> GAMAVKVARPCRKIEKWTYLELKGSKANEGVPQAMTAFAEFLNRTGIPINPRFSPGMSMSVPGSEKEFFAKVKELMSSHQFVV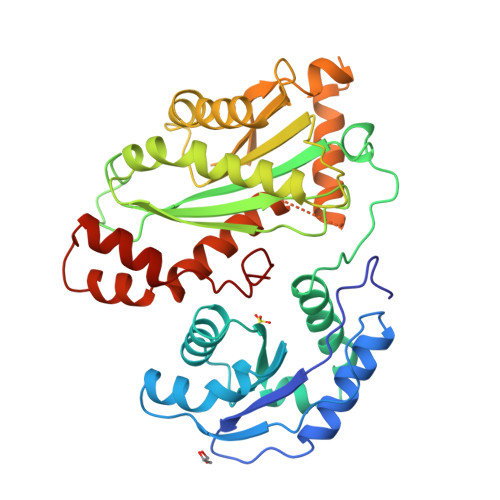VLLPRKDVAIYNMVKRAADITFGVHTVCCVAEKFLSTKGQLGYFANVGLKVNLKFGGTNHNIKTPIPLLAKGKTMVVGYDVTHPTNLAAGQSPASAPSIVGLVSTIDQHLGQWPAMVWNNPHGQESMTEQFTDKFKTRLELWRSNPANNRSLPENILIFRDGVSEGQFQMVIKDELPLVRAACKLVYPAGKLPRITLIVSVKGSGSAHYTVLVDEIFRADYGNKAADTLEQLTHDMCYLFGRATKAVSICPPAYYADLVCDRARIHQKELFDALDENDSVKTDDFARWGNSGAVHPNLRNSMYYI>[3x]MNQNLLVTKRDGSTERINLDKIHRVLDWAAEGLHNVSISQVELRSHIQFYDGIKTSDIHETIIKAAADLISRDAPDYQYLAARLAIFHLRKKAYGQFEPPALYDHVVKMVEMGKYDNHLLEDYTEEEFKQMDTFIDHDRDMTFSYAAVKQLEGKYLVQNRVTGEIYESAQFLYILVAACLFSNYPRETRLQYVKRFYDAVSTFKISLPTPIMSGVRTPTRQFSSCVLIECGDSLDSINATSSAIVKYVSQRAGIGINAGRIRALGSPIRGGEAFHTGCIPFYKHFQTAVKSCSQGGVRGGAATLFYPMWHLEVE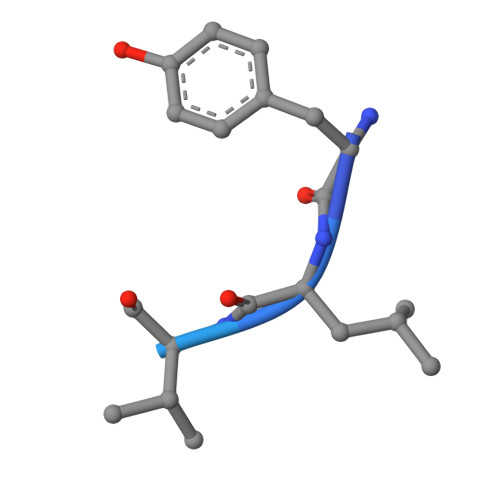SLLVLKNNRGVEGNRVRHMDYGVQINKLMYTRLLKGEDITLFSPSDVPGLYDAFFADQEEFERLYTKYEKDDSIRKQRVKAVELFSLMMQERASTGRIYIQNVDHCNTHSPFDPAIAPVRQSNLCLEIALPTKPLNDVNDENGEIALCTLSAFNLGAINNLDELEELAILAVRALDALLDYQDYPIPAAKRGAMGRRTLGIGVINFAYYLAKHGKRYSDGSANNLTHKTFEAIQYYLLKASNELAKEQGACPWFNETTYAKGILPIDTYKKDLDTIANEPLHYDWEALRESIKTHGLRNSTLSALMPSETSSQISNATNGIEPPRGYVSIKASKDGILRQVVPDYEHLHDAYELLWEMPGNDGYLQLVGIMQKFIDQSISANTNYDPSRFPSGKVPMQQLLKDLLTAYKFGVKTLYAQNTRDGAEDAQDDLVPSIQDDGCESGACKI;>YLVGQIDSEVDTDDLSNFQL[4x]> DLSKQMEEEAVRMFIEWLKNGGPSSGAP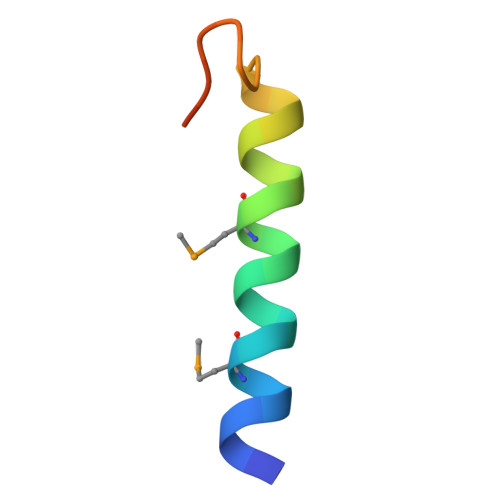PPS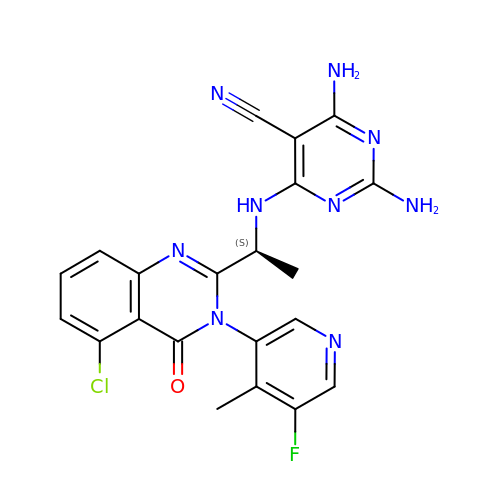2,4-bis(azanyl)-6-[[(1~{S})-1-[5-chloranyl-3-(5-fluoranyl-4-methyl-pyridin-3-yl)-4-oxidanylidene-quinazolin-2-yl]ethyl]amino]pyrimidine-5-carbonitrile | C21 H17 Cl F N9 O | UISOZEPWNXYPCK-JTQLQIEISA-N>MARRILSVLLENESGALSRVIGLFSQRGYNIESLTVAPTDDPTLSRMTIQTVGDEKVLEQIEKQLHKLVDVLRVSELGQGAHVEREIMLVKIQASGYGRDEVKRNTEIFRGQIIDVTPSLYTVQLAGTSG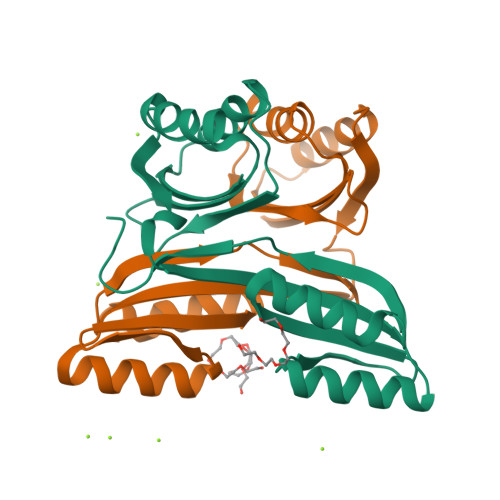KLDAFLASIRDVAKIVEVARSGVVGLSRGDKIMR[2x]> SNAMEKYQNLLVVIDPNQDDQPALRRAVYIVQRNGGRIKAFLPVYDLSYDMTTLLSPDERNAMRK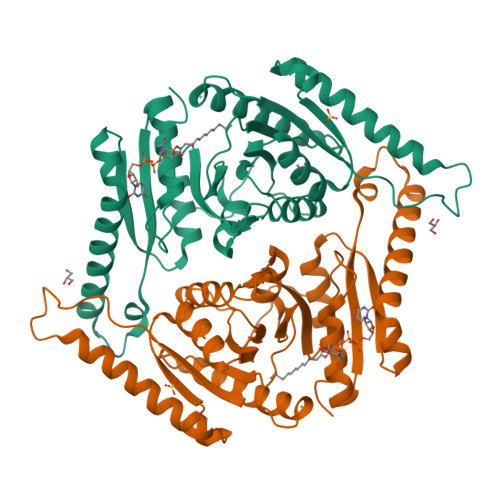GVINQKTAWIKQQARYYLEAGIQIDIKVIWHNRPYEAIIEEVITDKHDLLIKMAHQHDKLGSLIFTPLDWQLLRKCPAPVWMVKDKEWPEYGTIVVAANLSNEESYHDALNLKLIELTNDLSHRIQKDPDVHLLSAYPVAPINIAIELPDFDPNLYNNALRGQHLIAMKELRQKFSIPEEKTHVKEGLPEQVIPQVCEELNAGIVVLGILGRTGLSAAFLGNTAEQLIDHIKCDLLAIKPDGFTCPITVDSDNE>[2x]GSNSNEYRVRRERNNIAVRKSRDKAK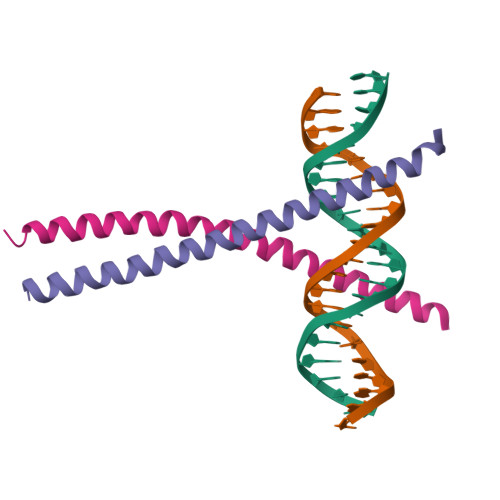QRNVETQQKVLELTSDNDRLRKRVEQLSRELDTLRG> GSHMEMAGDLSAGFFMEELNTYRQKQGVVLKYQELPNSGPPHDRRFTFQVIIDGREFPEGEGRSKKEAKNAAAKLAV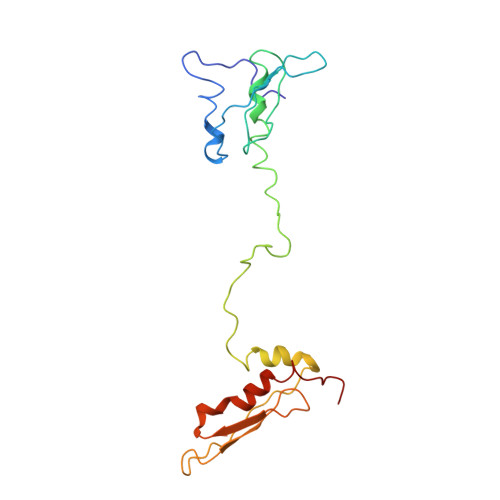EILNKEKKAVSPLLLTTTNSSEGLSMGNYIGLINRIAQKKRLTVNYEQCASGVHGPEGFHYKCKMGQKEYSIGTGSTKQEAKQLAAKLAYLQILSEETGSGC(2E)-3-{5-[(2,4-diaminopyrimidin-5-yl)methyl]-2,3-dimethoxyphenyl}-1-[(1S)-1-(propan-2-yl)phthalazin-2(1H)-yl]prop-2-en-1-one | C27 H30 N6 O3 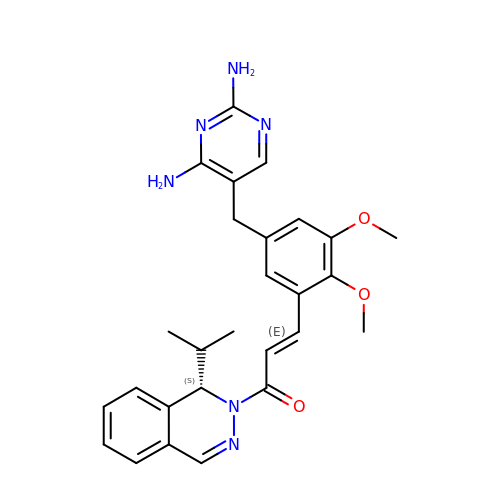| QGKBSLZXGYTSQX-GTCGAKFVSA-N>MTTRSAEHTTFVIERRLTAPVARVFRAWSTPESKRQWFACHGEWVPLEYALDFRPGGTERNYTADTDGLLHAYDARYIDIVPDTRIIYAYEMKLGQTRISASLVTVAFDVEPSGTRMVFTEQVVFLDGYGDNGARLQGT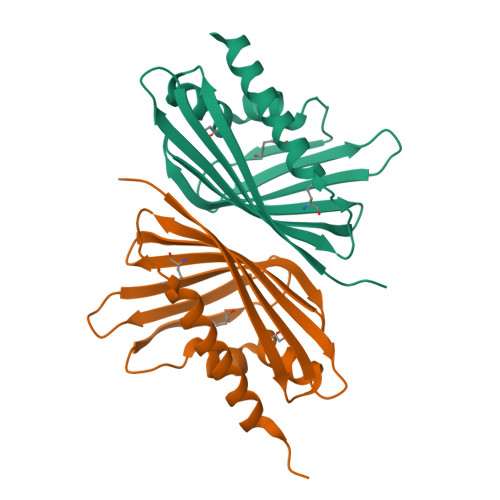EIGLDNLELFLVRETSPIHLEHHHHHH[2x]> MSEMTPREIVSELDQHIIGQADAKRAVAIALRNRWRRMQLQEPLRHEVTPKNILMIGPTGVGKTEIARRLAKLANAPFIKVEATKFTEVGYVGKEVDSIIRDLTDSAGGAIDAVEQNGIVFIDEIDKICKKGEYSGADVSREGVQRDLLPLVEGSTVSTKHGMVKTDHILFIASGAFQVARPSDLIPELQGRLPIRVELTALSAADFERILTEPHASLTEQYKALM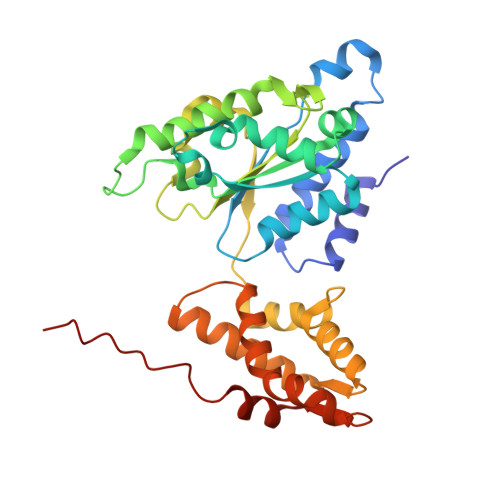ATEGVNIAFTTDAVKKIAEAAFRVNEKTENIGARRLHTVMERLMDKISFSASDMNGQTVNIDAAYVADALGEVVENEDLSRFIL>[2x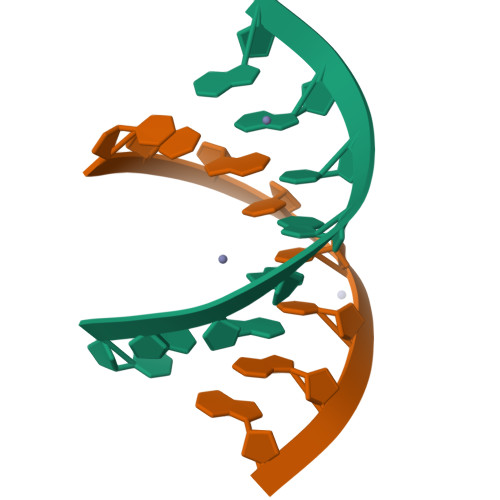]CUGGGCGG;>[2x]CCGCCUGG>MIPDDEFIKNPSVPGPTAMEVRCLIMCLAEPGKNDVAVDVGCGTGGVTLELAGRVRRVYAIDRNPEAISTTEMNLQRHGLGDNVTLMEGDAPEALCKIPDIDIAVVGGSGGELQEILRIIKDKLKPGGRIIVTAILLETKFEAMECLRDLGFDVNI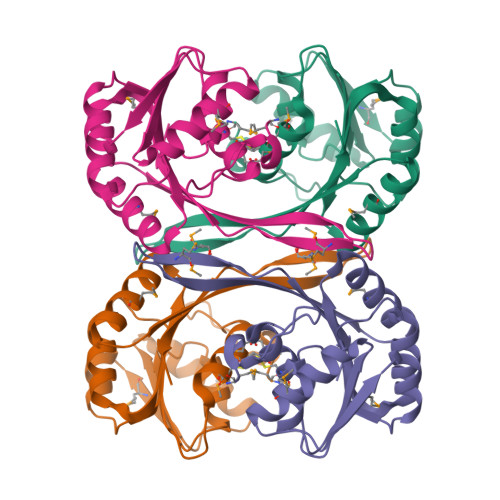TELNIARGRALDRGTMMVSRNPVALIYTGVSHENKD[4x]> MKVNMEYTKEKKVGEGTYAVVYLGCQHSTGRKIAIKEIKTSEFKDGLDMSAIREVKYLQEMQHPNVIELIDIFMAYDNLNLVLEFLPTDLEVVIKDKSILFTPADIKAWMLMTLRGVYHCHRNFILHRDLKPNNLLFSPDGQIKVADFGLARAIPAPHEILTSNVVTRWYRAPELLFGAKHYTSAIDIWSVGVIFAELMLRIPYLPGQNDVDQMEVTFRALGTPTDRDWPEVSSFMTYNKLQIYPPPSRDELRKRFIA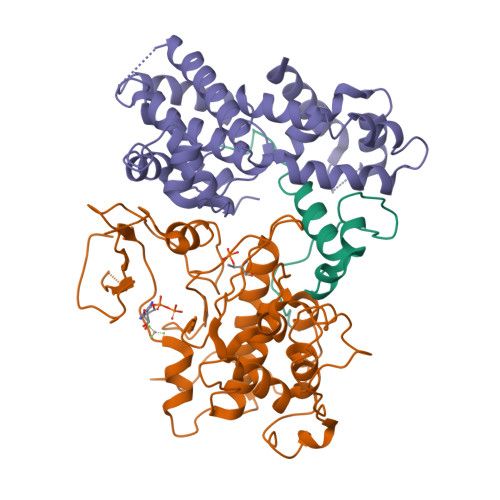ASEYALDFMCGMLTMNPQKRWTAVQCLESDYFKELPPPSDPSSIKIRN;> MTDIQLNGKSTLDTPSATMSAKEKEAKLKSADENNKPPNYKRISDSQLYRHSSQYRMWSYTKDQLQEKRVDTNARAIAYIEENLLKFREAHNLTEEEIKVLEAKAIPLTMEEELDLVNFYAKKVQVIAQHLNLPTEVVATAISFFRRFFLENSVMQIDPKSIVHTTIFLACKSENYFISVDSFAQKAKSTRDSVLKFEFKLLESLKFSLLNHHPYKPLHGFFLDIQNVLYGKVDLNYMGQIYDRCKKRITAALLTDVVYFYTPPQITLATLLIEDEALVTRYLETKFPSREGSQESVPGNEKEEPQNDASTTEKNKEKSTESEEYSIDSAKLLTIIRECKSIIEDCKPPSTEEAKKIAAKNYYCQNPSTLIQKLKRKLNGEDTSSTVEKKQKT;> MLMDEYEENKDMCPICKTDRYLSPDVKFLVNPECYHRICESCVDRIFSLGPAQCPYKGCDKILRKNKFKTQIFDDVEVEKEVDIRKRVFNVFNKTIDDFNGDLVEYNKYLEEVEDIIYKLDHGIDVAKTEEKLRTYEELNKQLIMNNLERSRTEIESFEQRQKFEKEMKLKKRLLERQIEEEERMNKEWTKKEIVNRLSTTTQDINETIEGVKNTVKLKKSSARRKLEELNRVLKNNPYFNSNVNVQNSRLKDAVPFTPFNGDREAHPPFTLKGSVYNDPFIKDLEHRKEFIASGFNTNYAYERVLTEAFMGLGCVISEEL>DYKDDDDKQSFSSSSSCTEEENKHHMGIDVIIKVTKQDQTPTNDKICQSVTEVTESEDESEEVVKGDPTTYYTVVGGGLTMDFGFTKCPKISSISEYSDGNTVNARLSSVSPGQGKDSPAITREEALS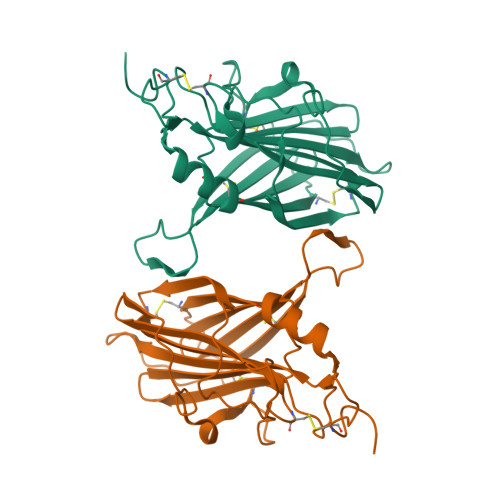MIKDCEMSINIKCSEEEKDSNIKTHPVLGSNISHKKVSYEDIIGSTIVDTKCVKNLEISVRIGDMCKESSELEVKDGFKYVDGSASEDAADDTSLINSAKLIACV[2x]>MVLYFIGLGLYDERDITV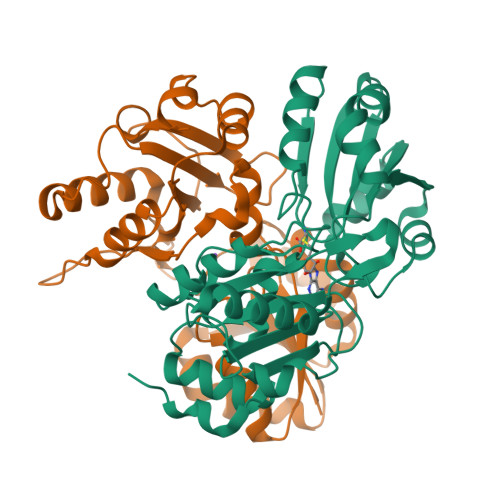KGLEIAKKCDYVFAEFYTSLMAGTTLGRIQKLIGKEIRVLSREDVELNFENIVLPLAKENDVAFLTPGDPLVATTHAELRIRAKRAGVESYVIHAPSIYSAVGITGLHIYKFGKSATVAYPEGNWFPTSYYDVIKENAERGLHTLLFLDIKAEKRMYMTANEAMEMLLKVEDMKKGGVFTDDTLVVVLARAGSLNPTIRAGYVKDLIREDFGDPPHILIVPGKLHIVEAEYLVEIAGAPREILRVNV[2x]>MKFAEHLSAHITPEWRKQYIQYEAFKDMLYSAQDQAPSVEVTDEDTVKRYFAKFEEKFFQTCEKELAKINTFYSEKLAEAQRRFATLQNELQSSLDAQKESTGVTTLRQRRKPVFHLSHEERVQHRNIKDLKLAFSEFYLSLILLQNYQNLNFTGFRKILKKHDKILETSRGADWRVAHVEVAPFYTCKKINQLISETEAVVTNELEDGDRQKAMKRLRVPPLGAAQPAPAWTTFRVGLFCGIFIVLNITLVLAAVFKLETDRSIWPLIRIYRGGFLLIEFLFLLGINTYGWRQAGVNHVLIFELNPRSNLSHQHLFEIAGFLGILWCLSLLACFFAPISVIPTYVYPLALYGFMVFFLINPTKTFYYKSRFWLLKLLFRVFTAPFHKVGFADFWLADQLNSLSVILMDLEYMICFYSLELKWDESKGLLPNNSEESGICHKYTYGVRAIVQCIPAWLRFIQCLRRYRDTKRAFPHLVNAGKYSTTFFMVTFAALYSTHKERGHSDTMVFFYLWIVFYIISSCYTLIWDLKMDWGLFDKNAGENTFLREEIVYPQKAYYYCAIIEDVILRFAWTIQISITSTTLLPHSGDIIATVFAPLEVFRRFVWNFFRL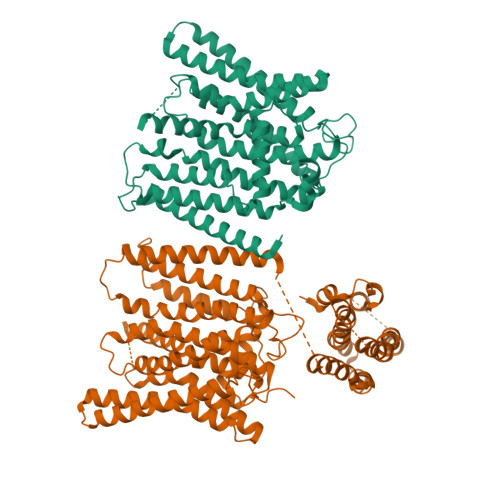ENEHLNNCGEFRA[2x]>[3x]XGEL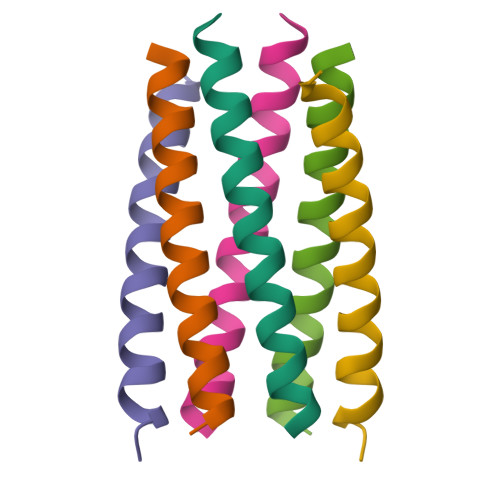AQALKELAKALKEQAWALKELAQALKGX> GLGQMLESMIDNTVRETVGAATSRDALPNTEASGPTHSKEIPALTAVETGATNPLVPSDTVQTRHVVQHRSRSESSIESFFARGACVTIMTVDNPASTTNKDKLFAVWKITYKDTVQLRRKLEFFTYSRFDMELTFVVTANFTETNNGHALNQVYQIMYVPPGAPVPEKWDDYTWQTSSNPSIFYTYGTAPARISVPYVGISNAYSHFYDGFSKVPLKDQSAALGDSLYGAASLNDFGILAVRVVNDPNPTKVTSKIRVYLKPKHIRVWCPRPPRAVAYYGPGVDYKDGT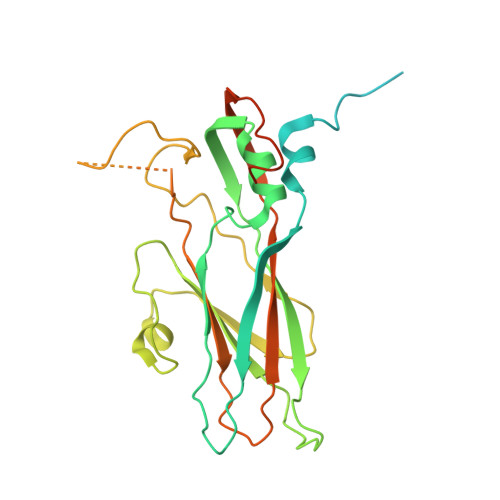LTPLSTKDLTTY>MHHHHHHHHHGGPISKILVANRSEIAIRVFRAANELGIKTVAIWAEEDKLALHRFKADESYQVGRGPHLARDLGPIESYLSIDEVIRVAKLSGADAIHPGYGLLSESPEFVDACNKAGIIFIGPKADTMRQLGNKVAARNLAISVGVPVVPATEPLPDDMAEVAKMAAAIGYPVMLKASWGGGGRGMRVIRSEADLAKEVTEAKREAMAAFGKDEVYLEKLVERARHVESQILGDTHGNVVHLFERDCSVQRRNQKVVERAPAPYLSEAQRQELAAYSLKIAGATNYIGAGTVEYLMDADTGKFYFIEVNPRIQVEHTVTEVVTGIDIVKAQIHILDGAAIGTPQSGVPNQEDIRLNGHALQCRVTTEDPEHNFIPDYGRITAYRSASGFGIRLDGGTSYSGAIITRYYDPLLVKVTAWAPNPLEAISRMDRALREFRIRGVATNLTFLEAIIGHPKFRDNSYTTRFIDTTPELFQQVKRQDRATKLLTYLADVTVNGHPEAKDRPKPLENAARPVVPYANGNGVKDGTKQLLDTLGPKKFGEWMRNEKRVLLTDTTMRDGHQSLLATRMRTYDIARIAGTYSHALPNLLSLECWGGATFDVSMRFLTEDPWERLALIREGAPNLLLQMLLRGANGVGYTNYPDNVVKYFVRQAAKGGIDLFRVFDCLNWVENMRVSMDAIAEENKLCEAAICYTGDILNSARPKYDLKYYTNLAVELEKAGAHIIAVKDMAGLLKPAAAKVLFKALREATGLPIHFHTHDTSGIAAATVLAAVEAGVDAVDAAMDALSGNTSQPCLGSIVEALSGSERDPGLDPAWIRRISFYWEAVRNQYAAFESDLKGPASEVYLHEMPGGQFTNLKEQARSLGLETRWHQVAQAYADANQMFGDIVKVTPSSKVVGDMALMMVSQDLTVADVVSPDREVSFPESVVSMLKGDLGQPPSGWPEALQKKALKG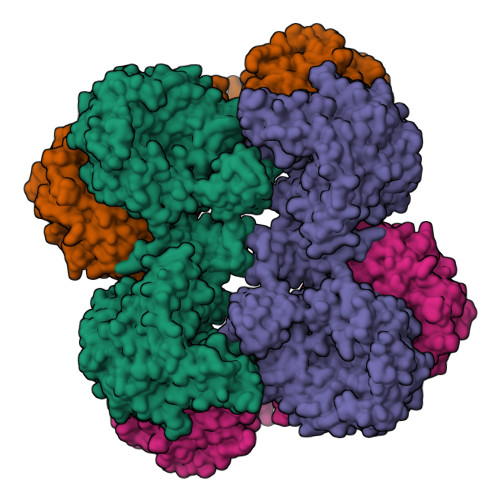EKPYTVRPGSLLKEADLDAERKVIEKKLEREVSDFEFASYLMYPKVFTDFALASDTYGPVSVLPTPAYFYGLADGEELFADIEKGKTLVIVNQAVSATDSQGMVTVFFELNGQPRRIKVPDRAHGATGAAVRRKAEPGNAAHVGAPMPGVISRVFVSSGQAVNAGDVLVSIEAMKMETAIHAEKDGTIAEVLVKAGDQIDAKDLLAVYGG[2x]>THLNTYESVTPDPDVDVIIIGAGISGSAAAKALHDQGASVLVVEANDRIGGRTWTEQEGAPGGPIDYGGMFIGETHTHLIELGTSLGLEMTPSGKPGDDTYIVAGNVLRAPDDQLDPNLPFVPEFLSSLKALDELADSVGWDQPWASPNAAALDSKTVATWLAETIESEEVRRLHTVIVNTLLGADPYEVSLLYWAYYVSECEGIQSLMGTRDGAQWAWWFGGAAQVSWRIADAIGRDKFLLEWPVDRIEHDESGVTLFSGQRSLRARHIVIAMSPLAANQIRFEPALPTSRAQLQARAPMGRYYKVQARYPSSFWVEQGYSGALLDTEDVGVFLLDGTKPTDTLATLIGFIGGSNYDRWAAHTPQERERAFLDLLVKAFGPQAADPSYFHETDWTQQEWAKGGPVTYMPPGVLANFGAALRDPVGKVHFAGTEASFQWSGYMEGGVRAGQKAAAAIAEELERTANKGALV[4x]

Originally described in B. oxydans strain IH-35A, CHAO carries out the initial step in the biodegradation pathway of cyclohexylamine, a high volume chemical used industrially as a corrosion inhibitor and in the rubber and water treatment industries. The CHAO structure can be divided into two domains: a cofactor-binding domain composed of two four-stranded β-sheets (one parallel, one mixed) and seven α-helices, and a substrate-binding domain consisting of a twisted seven-stranded mixed β-sheet and eight α-helices. The active site of CHAO is located in a buried cavity located at the interface of the substrate- and cofactor-binding domains. An examination of the three dimensional atomic structure of CHAO reveals that the overall fold is substantially similar to that of the human MAO B monomer, with a RMSD of 1.1 Å for the coordinates of the α-carbon atoms.

In order to determine the holoenzyme structure of CHAO, we employed molecular replacement using the A chain from human MAO B (30% sequence identity), truncated to remove the C-terminal predicted transmembrane helical segment, as a search model. Four molecules of CHAO were identified per asymmetric unit. Most of the polypeptide chain could be modeled into the electron density maps: residues 30–480 in the case of the holoenzyme and residues 30–478 in the ternary complex. For the apoenzyme structure, 90% of the residues fall into the favored region of a Ramachandran plot and 2.2% are outliers. When superimposed, the structures of CHAO crystallized with and without substrate present are very similar (RMSD 0.26 Å), with no significant differences in the positioning of secondary structural elements and with only minor differences in the conformation of loop regions. The structures of the CHAO holoenzyme and complex with cyclohexanone are remarkably similar, suggesting that there are no significant conformational changes associated with the binding of product in the active site. One side of this cavity is occupied by the flavin cofactor, held in place by hydrogen bonds and Van der Waals interactions with the protein. The isoalloxazine ring of the FAD cofactor is planar, and a lysine residue that is hydrogen bonded to the N5 atom of FAD in other MAOs (via a water molecule) is positioned to play that role in CHAO. In addition to the substrate-binding cavity, CHAO has a second cavity located closer to the protein surface that is shielded from the bulk solvent by a loop of the polypeptide chain (residues 128–138). This intermediate cavity is separated from the substrate-binding cavity by a series of amino acid side chains (T198, L199, M226, and F351).>MGSSHHHHHHSQDPNSMPDNTIQWDKDADGIVTLTMDDPSGSTNVMNEAYIESMGKAVDRLVAEKDSITGVVVASAKKTFFAGGDVKTMIQARPEDAGDVFNTVETIKRQLRTLETLGKPVVAAINGAALGGGLEIALACHHRIAADVKGSQLGLPEVTLGLLPGGGGVTRTVRMFGIQNAFVSVLAQGTRFKPAKAKEIGLVDELVATVEELVPAAKAWIKEELKANPDGAGVQPWDKKGYKMPGGTPSSPGLAAILPSFPSNLRKQLKGAPMPAPRAILAAAVEGAQVDFDTASRIESRYFASLVTGQVAKNMMQAFFFDLQAINAGGSRPEGIGKTPIKRIGVLGAGMMGAGIAYVSAKAGYEVVLKDVSLEAAAKGKGYSEKLEAKALERGRTTQERSDALLARITPTADAADFKGVDFVIEAVFENQELKHKVFGEIEDIVEPNAILGSNTSTLPITGLATGVKRQEDFIGIHFFSPVDKMPLVEIIKGEKTSDEALARVFDYTLAIGKTPIVVNDSRGFFTSRVIGTFVNEALAMLGEGVEPASIEQAGSQAGYPAPPLQLSDELNLELMHKIAVATRKGVEDAGGTYQPHPAEAVVEKMIELGRSGRLKGAGFYEYADGKRSGLWPGLRETFKSGSSQPPLQDMIDRMLFAEALETQKCLDEGVLTSTADANIGSIMGIGFPPWTGGSAQFIVGYSGPAGTGKAAFVARARELAAAYGDRFLPPESLLS[2x];>[2x]MSEEAFIYEAIRTPRGKQKNGSLHEVKPLSLVVGLIDELRKRHPDLDENLISDVILGCVSPVGDQGGDIARAAVLASGMPVTSGGVQLNRFCASGLEAVNTAAQKVRSGWDDLVLAGGVESMSRVPMGSDGGAMGLDPATNYDVMFVPQSIGADLIATIEGFSREDVDA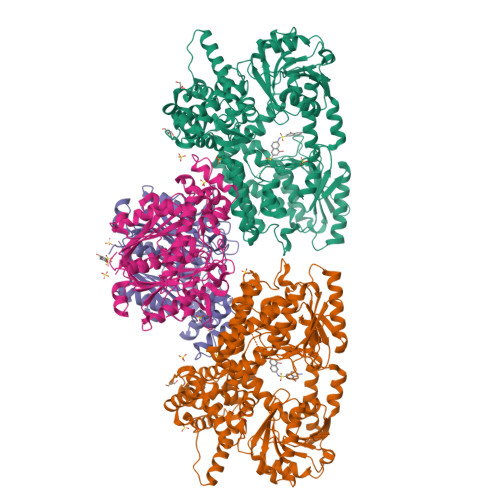YALRSQQKAAEAWSGGYFAKSVVPVRDQNGLLILDHDEHMRPDTTKEGLAKLKPAFEGLAALGGFDDVALQKYHWVEKINHVHTGGNSSGIVDGAALVMIGSAAAGKLQGLTPRARIVATATSGADPVIMLTGPTPATRKVLDRAGLTVDDIDLFELNEAFASVVLKFQKDLNIPDEKLNVNGGAIAMGHPLGATGAMILGTMVDELERRNARRALITLCIGGGMGVATIIERV> SRKIIHVDMDCFFAAVEMRDNPALRDIPIAIGGSRERRGVISTANYPARKFGVRSAMPTGMALKLCPHLTLLPGRFDAYKEASNHIREIFSRYTSRIEPLSLDEAYLDVTDSVHCHGSATLIAQEIRQTIFNELQLTASAGVAPVKFLAKIASDMNKPNGQFVITPAEVPAFLQTLPLAKIPGVGKVSAAKLEAMGLRTCGDVQKCDLVMLLKRFGKFGRILWERSQGIDERDVNSERLRKSVGVERTMAEDIHHWSECEAIIERLYPELERRLAKVKPDLLIARQGVKLKFDDFQQTTQEHVWPRLNKADLIATARKTWDERRGGRGVRLVGLHVTLLD;> RKIIHVDMDCFFAAVEMRDNPALRDIPIAIGGSRERRGVISTANYPARKFGVRSAMPTGMALKLCPHLTLLPGRFDAYKEASNHIREIFSRYTSRIEPLSLDEAYLDVTDSVHCHGSATLIAQEIRQTIFNELQLTASAGVAPVKFLAKIASDMNKPNGQFVITPAEVPAFLQTLPLAKIPGVGKVSA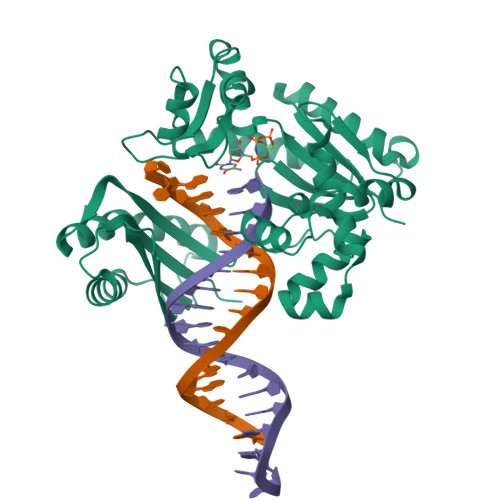AKLEAMGLRTCGDVQKCDLVMLLKRFGKFGRILWERSQGIDERDVNSERLRKSVGVERTMAEDIHHWSECEAIIERLYPELERRLAKVKPDLLIARQGVKLKFDDFQQTTQEHVWPRLNKADLIATARKTWDERRGGRGVRLVGLHVTLD> MSAEKLFTPLKVGAVTAPNRVFMAPLTRLRSIEPGDIPTPLMGEYYRQRASAGLIISEATQISAQAKGYAGAPGLHSPEQIAAWKKITA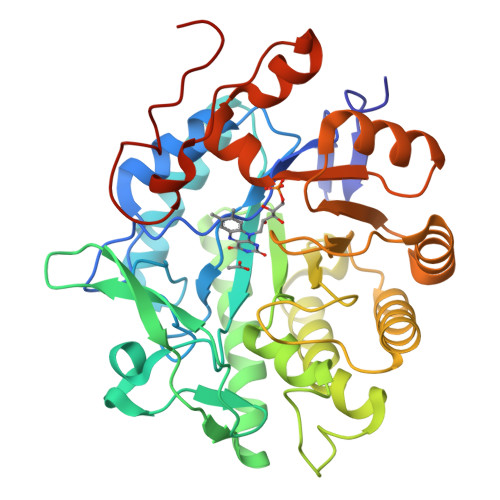GVHAEDGRIAVQLWHTGRISHSSIQPGGQAPVSASALNANTRTSLRDENGNAIRVDTTTPRALELDEIPGIVNDFRQAVANAREAGFDLVELHSAHGYLLHQFLSPSSNQRTDQYGGSVENRARLVLEVVDAVCNEWSADRIGIRVSPIGTFQNVDNGPNEEADALYLIEELAKRGIAYLHMSETDLAGGKPYSEAFRQKVRERFHGVIIGAGAYTAEKAEDLIGKGLIDAVAFGRDYIANPDLVARLQKKAELNPQRPESFYGGGAEGYTDYPSLHHHHHHHH The proteins MakA/B/E can form a tripartite toxin that lyses erythrocytes and is cytotoxic to cultured human cells. Here, we identify the proteins from the five V. cholerae genes, vca0880 through vca0884, that are coexpressed from the operon makDCBAE and analyze the crystal structures of MakA, MakB, and MakE. For structural analyses, MakA, MakB, and MakE were crystallized in their soluble, compact forms in which the hydrophobic β-tongue is hidden in the interface between their respective head and tail domain. Each protein is predicted to undergo a conformational change in which the head domain is unfolded and rearranged into two long helices in order to assemble into a membrane-bound tripartite complex.

MakB and MakE were refined to 2.1 and 2.0 Å resolution, respectively. MakE is structurally very similar to MakA, with a root mean square deviation of 2.3 Å calculated on 329 aligned Cα atoms. Its tail domain, 85 Å in length, consists of five long helices (α1, α2, α3, α6, and α7). The head domain, 55 Å in length, comprises two parallel helices (α4 and α5) and a four-stranded antiparallel β-sheet (strand order β1β5β2β6). β1 is very short and originates from the tail domain. MakE also has a β-hairpin (β3β4) protruding 90° from the sheet. Two molecules of MakE are found in the asymmetric unit, along with two nickel ions and four sulfate ions. MakE, which has the most prominent break of the α2-helix, has no proline at this position. In contrast, the hydrophobic region in MakE constitutes the first central β-strand (β2), the β-hairpin β3β4, and half of the next β-strand (β5). Similarly, an elongated form of MakE was modeled in which the tip of the long α3/α4 helices is hydrophobic, albeit the hydrophobic residues are more concentrated on one side. MakE, with its shorter β-tongue, can penetrate only a single membrane leaflet.

>[2x]GAMNQSASEQLQTDIPASISAMVLLNSACQGVVETYIDQGNAEHWYAQVEQNLNAVQKLVRQWRLSGNLYFSNDIMDSVLSIANTFKDSNVQILTLFKALETRFDTAQLQQLTSLILTLQNPIQSLTSNIKRYDEGLNAWARQVEDAHNTLQQTIAQIQQEEVSIQAEIIATNAQIDLMKQQIAAFKTAIANAQSQRKKGIFETIFGVVLAPFTLGGSLILAGFGVSSIVEAQSEISSLQSDIQSSLNTINHDQQTLSQDQQQIASLNALLLSVDQVNNDCAAISRSLDTLQTTVLSLYNETNNVVSNLTKAQDSQAVILEQVWYQSAYNEWQDILEVASTLNNAQPQITKAQIK>GDNQDRTVANTQPSGPSNSTEIPALTAVETGHTSQVDPSDTIQTRHVVNFHSRSESTIENFMGRAACVFMDQYKINGEETSTDRFAVWTINIREMAQLRRKCEMFTYMRFDIEMTMVITSCQDQGTILDQDMPVLTHQIMYVPPGGPIPAKVDGYEWQTSTNPSVFWTEGNAPPRISIPFISVGNAYSSFYDGWSHFTQDGTYGYTTLNAMGKLYIRHVNRSSPHQITSTIRVYFKPKHIKAWVPRPPRLCPYINKRDVNFVVTEITDSRTSITDTPHPEHSVLATH[11x];>SPSAEECGYSDRVRSMTLGNSTITTQESANVVVGYGEWPSYLSDREATAEDQPTQPDVATCRFYTLESVQWEKTSPGWWWKFPEALKNMGLFGQNMHYHYLGRAGYTIHVQCNASKFHQGCLLVVCVPEAEMGCADTDTTFPATELTTEDTPHVFTSDSITGKKVQAAVCNAGMGVGVGNLTIFPHQWINLRTNNSATIVIPYINSVPMDNMFRHYNFTLMIIPFAPLNFTDGATAYVPITVTIAPMYAEYNGLRLAST[11x];>GVPVLNTPGSNQFLTSDDYQSPSAMPQFDETPEMHIPGEVRNLMEIAEVDSVVPVNNVTGKTKSMDAYQIPVGTGNTDKTKPIFSFQMDPGYSSVLKRTLLGEMLNYYAHWSGSVKL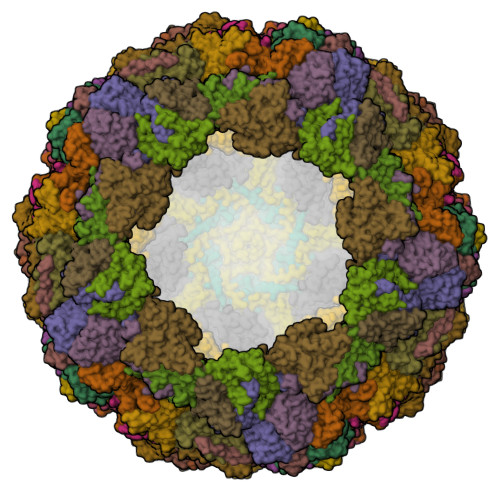TFLFCGSAMATGKLLISYSPPGASVPTSRKDAMLGTHIVWDIGLQSSCVLCVPWISQSHYRMVQQDPYTSAGYITCWYQTNIVVPPGAPTSCDVLCFASACNDFSVRLLRDTPFMAQPGKLQ[11x]>MAELPTTETPGDATLCSGRFTISTLLSSDEPSPPAAYDSSHPSHLTHSSTFCMRDFGYNDIDVVPTYEHYANDTQPGEPRKVRPTLADLHSFLKQEGRHLHALAFDSRPSHEMTDGLVEGEAGTSSEKNPEEPVRFGWVNGVMIRCMLNIWGVILYLRLPWITAQAGIVLTWIIILLSVTVTSITGLSISAISTNGKVKSGGTYFLISRSLGPELGGSIGLIFAFANAVGVAMHTVGFAETVRDLLQEYGAPIVDPINDIRIIGVVSVTVLLAISLAGMEWESKAQVLFFLVIMVSFANYLVGTLIPPSEDKASKGFFSYRADIFVQNLVPDWRGPDGTFFGMFSIFFPSATGILAGANISGDLKDPAIAIPKGTLMAIFWTTISYLAISATIGSCVVRDASGVLNDTVTPGWGACEGLACSYGWNFTECTQQHSCHYGLINYYQTMSMVSGFAPLITAGIFGATLSSALACLVSAAKVFQCLCEDQLYPLIGFFGKGYGKNKEPVRGYLLAYAIAVAFIIIAELNTIAPIISNFFLCSYALINFSCFHASITNSPGWRPSFQYYNKWAALFGAIISVVIMFLLTW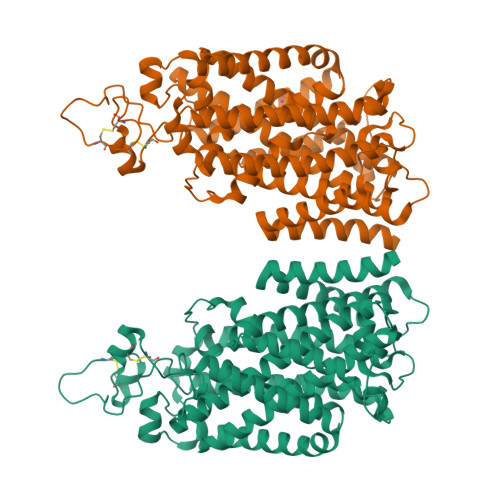WAALIAIGVVLFLLLYVIYKKPEVNWGSSVQAGSYNLALSYSVGLNEVEDHIKNYRPQCLVLTGPPNFRPALVDFVGTFTRNLSLMICGHVLIGPHKQRMPELQLIANGHTKWLNKRKIKAFYSDVIAEDLRRGVQILMQAAGLGRMKPNILVVGFKKNWQSAHPATVEDYIGILHDAFDFNYGVCVMRMREGLNVSKMMQAHINPVFDPAEDGKEASARVDPKALVKEEQATTIFQSEQGKKTIDIYWLFDDGGLTLLIPYLLGRKRRWSKCKIRVFVGGQINRMDQERKAIISLLSKFRLGFHEVHILPDINQNPRAEHTKRFEDMIAPFRLNDGFKDEATVNEMRRDCPWKISDEEITKNRVKSLRQVRLNEIVLDYSRDAALIVITLPIGRKGKCPSSLYMAWLETLSQDLRPPVILIRGNQENVLTFYCQ[2x]> MTVPLYKQIASLIEDSIVDGTLSIDQRVPSTNELA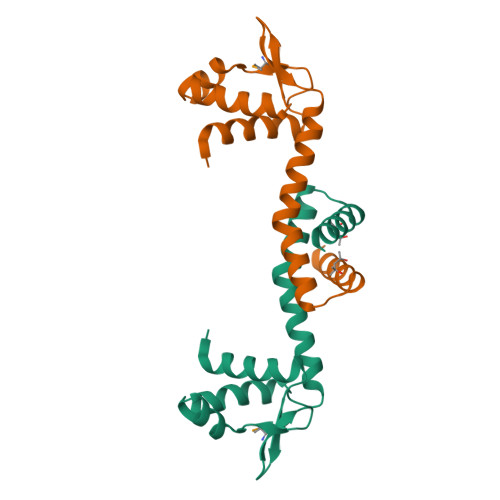AFHRINPATARNGLTLLVEAGILYKKRGIGMFVSAQAPALIRERRDAAFAATYVAPLIDESIHLGFTRARIHALLDQVAESRGLYKLEHHHHHH>[2x]MGSIGEPNRLLCWSIYVTKKPDQSEEDHHNHVSKVNAPMFIPFLKKYGIVRYTVKHNDAYSKPKQAALMAGQPEE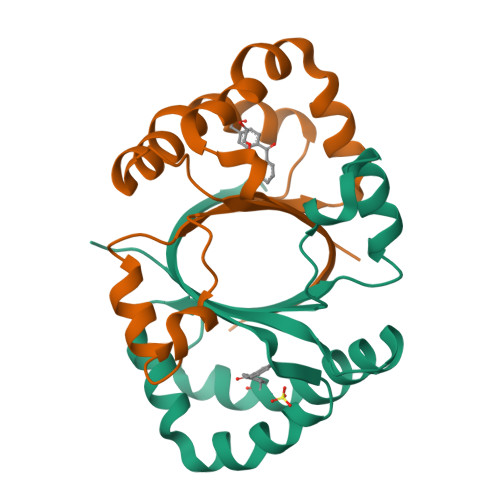NVLAYDTVFEMIVKDIESIQTMQKDEEFLRTTIPDHFNFADMTRSKGSLTWIEEFTFALEHHHHHH> LSDSRVLWAPAEAHPLSPQGHPARLHRIVPRLRDVFGWGNLTCPICKGLFTAINLGLKKEPNVARVGSVAIKLCNLLKIAPPAVCQSIVHLFEDDMVEVWRRSVLSPSEACGLLLGSTCGHWDIFSSWNISLPTVPKPPPKPPSPPAPGAPVSRILFLTDLHWDHDYLEGTDPDCADPLCCRRGSGLPPASRPGAGYWGEYSKCDLPLRTLESLLSGLGPAGPFDMVYWTGDIPAHDVWHQTRQDQLRALTTVTALVRKFLGPVPVYPAVGNHESTPVNSFPPPFIEGNHSSRWLYEAMAKAWEPWLPAEALRTLRIGGFYALSPYPGLRLISLNMNFCSRENFWLLINSTDPAGQLQWLVGELQAAEDRGDKVHIIGHIPPGHCLKSWSWNYYRIVARYENTLAAQFFGHTHVDEFEVFYDEETLSRPLAVAFLAPSATTYIGLNPGYRVYQIDGNYSGSSHVVLDHETYILNLTQANIPGAIPHWQLLYRARETYGLPNTLPTAWHNLVYRMRGDMQLFQTFWFLYHKGHPPSEPCGTPCRLATLCAQLSARADSPALCRHLMPDGSLPEAQSLWPRPLFC

ASMD is a result of mutations in acid sphingomyelinase (ASM, E.C. 3.1.4.12), which hydrolyzes sphingomyelin to ceramide and phosphocholine. The structure includes an N-terminal saposin domain (residues 84–167), a proline-rich linker (168–195), a catalytic metallophosphatase domain (196–538), and a helical C-terminal domain (539–611). The substrate binding cleft in ASM is created by the catalytic domain in the middle, and saposin domain and C-terminal domain at two opposite sides. Zinc ions are prerequisites for activity of both forms.

Full-length human ASM was expressed from HEK293S N-acetylglucosaminyl transferase I-deficient (Gnt1−) cells with Man5 type glycans. Purified protein was crystallized at pH 5.5. Therefore, the holoenzyme structure was determined using single-wavelength anomalous diffraction (SAD) from a Pt derivative at 2.43 Å, and the phases was extended to 2.25 Å using a Zn-SAD data set. The final model was refined to Rfree of 0.203. Clear electron density allowed us to build all residues from W84 to M611 as well as two zinc ions, six N-linked glycans, and eight disulfides. Two neighbouring zinc ions are identified in the center of the cleft. The two zinc ions are separated by 3.5 Å and referred to as Zn1 and Zn2. D278 bridges between Zn1 and Zn2 at the axial positions, while H457 and H459 are in the other axial positions. The precise side-chain arrangement around the metals facilitates recruitment of a key catalytic water molecule to the third equatorial position bridging between Zn1 and Zn2. The catalytic water is stabilized and positioned by hydrogen bonds to the main chain carbonyl of H457.There is an asymmetric arrangement in which the carboxylate oxygen of D278 is slightly closer to Zn2 (D-Zn1 2.5 Å, D-Zn2 1.9 Å), while the catalytic water is closer to Zn1 (Wat-Zn1 1.9 Å, Wat-Zn2 2.6 Å).>[2x]MPIHIGSSIPLMVEKMLTEMVKPSKHIPQQTLNLSTLDNDPYNEVIYKACYVFKAKNVADDDNRPEALLREALSDLLGYYYPLSGSLKRQESDRKLQLSCGGDGGGVPFTVATANVELSSLKNLENIDSDTALNFLPVLHVDIDGYRPFALQVTKFECGGFILGMAMSHAMCDGYGEGHIMCALTDLAGGKKKPMVTPIWERERLVGKPEDDQPPFVPGDDTAASPYLPTDDWVTEKITIRADSIRRLKEATLKEYDFSNETITTFEVIGAYLWKSRVKALNLDRDGVTVLGLSVGIRNVVDPPLPDGYYGNAYIDMYVPLTAREVEEFTISDIVKLIKEAKRNAHDKDYLQEELANTEKIIKMNLTIKGKKDGLFCLTDWRNIGIFGSMDFGWDEPVNIVPVVPSETARTVNMFMRPSRLESDMVGGVQIVVTLPRIAMVKFKEEMEALE

Phenolamides, also known as phenylamides or hydroxycinnamic acid amides, are ubiquitous secondary metabolites in plants. All these phenolamide synthesis enzymes belong to the acyl-coenzyme A (CoA)-dependent BAHD acyltransferases family, which was named according to the first letter of each of its first four biochemically characterized enzymes: Benzylalcohol O-acetyltransferase, Anthocyanin O-HCT, HCT of anthranilate, and Deacetylvindoline 4-O-acetyltransferase. It has been established that BAHD acyltransferases catalyze the transfer of acyl groups from acyl-donors (Acyl-CoA) to various acyl-acceptors. In this study, we first performed structural analyses on two representative BAHD family enzymes, the Arabidopsis mono-/di-acyltransferase-SDT (AtSDT) and poly acyltransferase-SHT (AtSHT), then explored the acceptor-molecule specificity and potential molecular mechanisms of multisite acylation by structure-based mutagenesis approaches, and, finally, successfully predicted and varified the acyl acceptor substrates of two uncharacterized BAHD family transferases in Arabidopsis using our prediction methods on the basis of a sequence similarity network (SSN) and of structure modeling.

Spermidine disinapoyl/dicoumaroyl transferases AtSDT and AtSCT were expressed mainly in the seed and root of Arabidopsis.>AAMKVYDVTAPIYEGMPVYKNKPEKQPKRTTITNGYVTESRIDMDVHTGTHIDAPLHMVEGGATFETIPLNDLVGPCKLFDLTHVNDRITKDDIAHLDIQEGDFVLFKTKNSFEDAFHFEFIFVAEDAARYLADKQI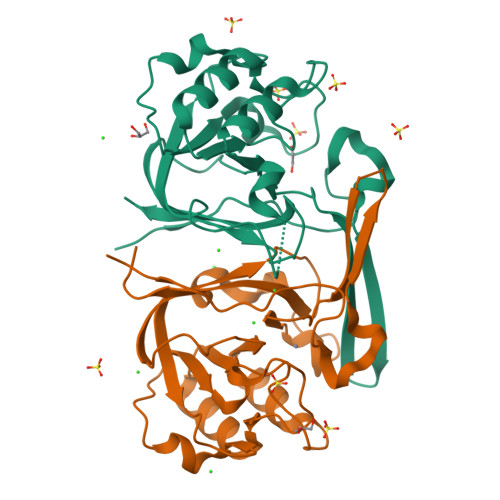RGVGIDALGIERAQEGHPTHKTLFSAGVIIIEGLRLKDVPEGRYFMVAAPLKLVGTDAAPARVLLFDREP[2x]> MEDLCVANTLFALNLFKHLAKASPTQNLFLSPWSISSTMAMVYMGSRGSTEDQMAKVLQFNEVGAAADKIHSSFRSLSSAINASTGNYLLESVNKLFGEKSASFREEYIRLCQKYYSSEPQAVDFLECAEEARKKINSWVKTQTKGKIPNLLPEGSVDGDTRMVLVNAVYFKGKWKTPFEKKLNGLYPFRVNSAQRTPVQMMYLREKLNIGYIEDLKAQILELPYAGDVSMFLLLPDEIADVSTGLELLESEITYDKLNKWTSKDKMAEDEVEVYIPQFKLEEHYELRSILRSMGMEDAFNKGRANFSGMSERNDLFLSEVFHQAMVD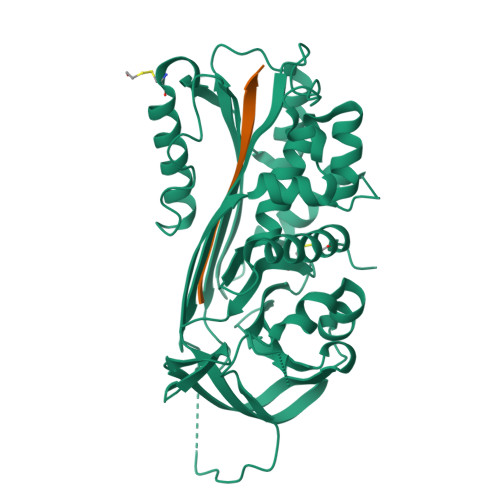VNEEGTEAAAGTGGVMTGRTGHGGPQFVADHPFLFLIMHKITNCILFFGRFSSP;> XTEAAAGTGGVMTGR>[2x]MENTENSVDSKSIKNLEPKIIHGSESMDSGISLDNSYKMDYPEMGLCIIINNKNFHKSTGMTSRSGTDVDAANLRETFRNLKYEVRNKNDLTREEIVELMRDVSKEDHSKRSSFVCVLLSHGEEGIIFGTNGPVDLKKIFNFFRGDRCRSLTGKPKLFIIQACRGTELDCGIETDSGVDDDMACHKIPVEADFLYAYSTA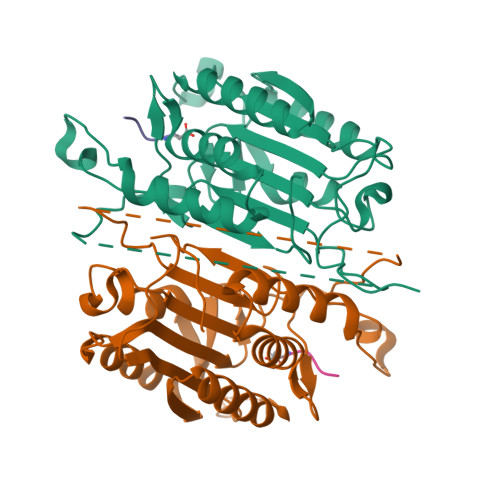PGYYSWRNSKDGSWFIQSLCAMLKQYADKLEFMHILTRVNRKVATEFESFSFDATFHAKKQIPCIVSMLTKELYFYH>[6x]SNAMTTKRVKKMGKEEMKEMFDLVIYAFNQEPTAERQERFEKLLSHTQSYGFLIDEQLTSQVMATPFQVNFHGVRYPMAGIGYVASYPEYRGEGGISAIMKEMLADLAKQKVALSYLAPFSYPFYRQYGYEQTFEQAEYTIKTEDWPRVKRVPGTIKRVSWADGKEVIKDVYLENQRAHSGGVIRETWWLDYTLNRASKPNNQAIYYSSEGKAEGYVIYRIAAGTFEIVEWNYLTNT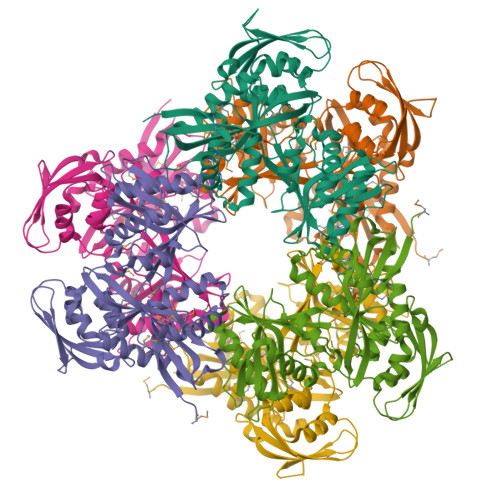AFKALAGFIGSHSGSVQSFHWINGFAGKDLNDLMPTPAASVKILPYMMARIVELQTFLEKYPFQSGEKETYSLEIEDSYGPWNEGIWTITIDEQGKATVTKGAAEKEGTAALKADIQTWTQLFLGYRSAETLSFYERLQGDATIAQRLGQRLVKGMPILEDYF> MAASKMNPVGNLLSTVSSTVGSLLQNPSVEEKEMDSDRVAASTTTNAGNLVQASVAPTMPVKPDFKNTDDFLSMSYRSTTAPTNPTKMVHLAHGTWTTNQHRQALVASITLLQAFWPNQDFPAWGQSRYFAAVRCGFHIQVQLNVNIGSAGCLIAAYMPKTAHDHMNTYTFGSYTNLPHVLMNAATTSQADLYIPYVFNHNYARTDSDDLGGIYIWVWSALTVPSGSPTTVDV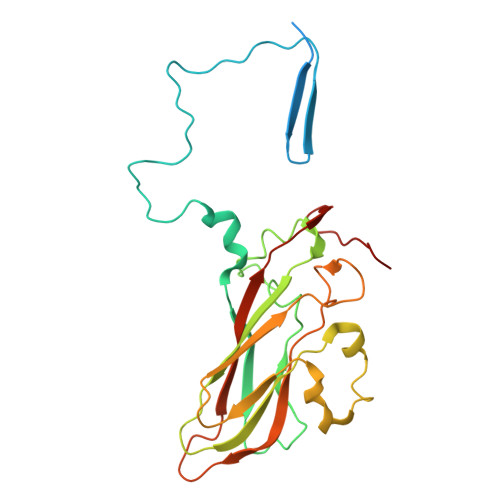TIFGSLLDLDFQCPRPPGADTVIYTQ> IDYLDASLRKKNKQRLKAI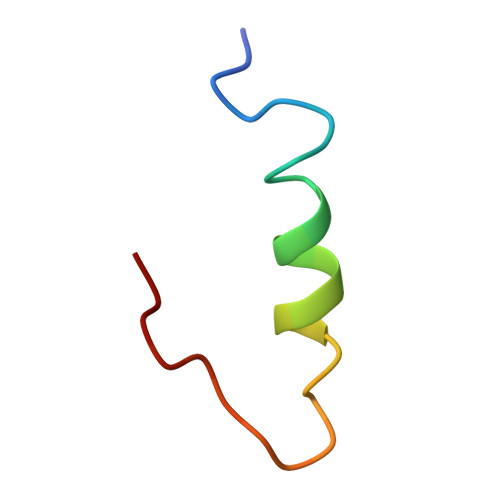QQGRQPQYLL> MLFFSFFKTLVDQEVVVELKNDIEIKGTLQSVDQFLNLKLDNISSTDEKKYPHLGSVRNIFIRGSTVRYVYLNKNMVDTNLLQD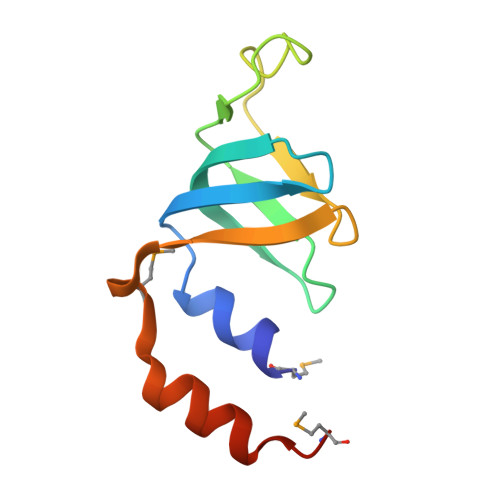ATRREVMTERK>MEMENKRSTQKVSRSIPERVKSALWSITAGRCEICCKKLYISDVTGSLVNISQMAHIKAFSPKGPRYSDEENNPHQLDNLLLLCAEHHKMIDTD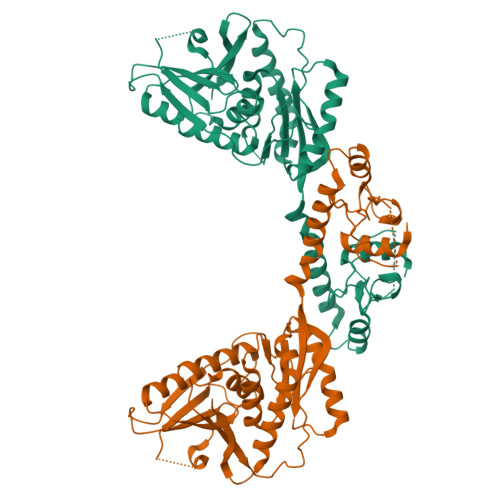PDDFPVDWLIKQKKEFEEKVDAVIDTQRIKSSILSFNSIITKNDEIKNEEAEFPKVLLFNDNYFDGNIYRINNALSGIEHDPMYYDLMCQSMKQQIEKIKIPLNSSETISVFAIAPQPLLLYLGYLLNDETNIKIYQRFRTGNLKWNWESSEITNNFYVEQLYTDGNEIDTEVNLILSLSAEISLDRIPTFSNQEYKVPTLILRSDRQGFDAIKSNEDVNEYISVFRNLVVEKIRNDFPNLKCINIFPATPVSVPVRMGMNYQKNIDVEWKIFNQQTNVGFIYSLSLKGEV[4x]> QPPLAPGLSFDFYKRSCPKAESIVRSFVQDAVRRDVGLAAGLLRLHFHDCFVQGCDASVLLDGSATGPGEQQAPPNLTLRPTAFKAINDIHDRLHKECGGTVVSCSDVLALAARDSVVVSGGPSYRVPLGRRDSASFATQQDVLSGLPPPTAAVPALLAVLSKINLDATDLVALSGGHTIGLGHCTSFEDRLFPRPDPTLNATFAGQLRRTCPAKGTDRRTPLDVRTPNAFDNKYY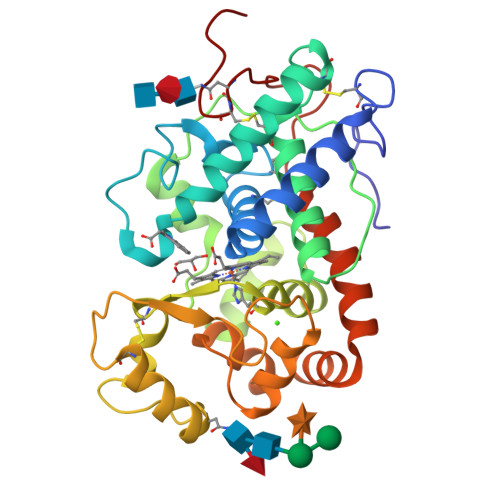VNLVNREGLFTSDQDLFSNARTRALVDKFARSQRDFFDQFAFSVVKMGQIKVLTGTQGQIRTNCSARNAAG>[4x]MNYGITESVKTTRSKIKIKDIVSDVVEKKANAIKYFLEGEEFKQAIVFGAYLSGSYIAYSLLKDCEEVIIVDIQPHLKDILFNDGIKFMDLNKLQLELRNGTSINPDLVIDLTGIGGVSPDLISKFNPKVLIVEDPKGNHDKGISKIDNTDKRLCVGAKKGV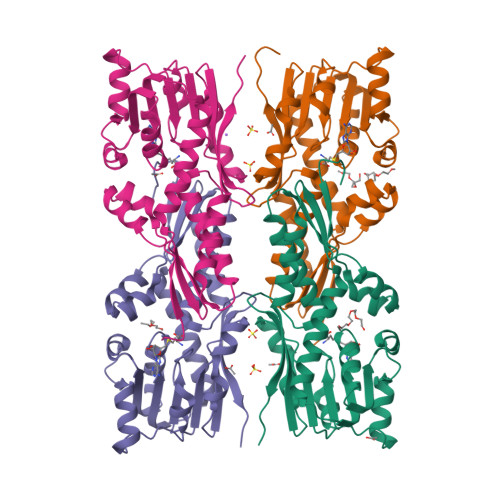LKTYRSSKFSKTSGTMTLVVDIIMDSCREINELDSVLYTIPNLKYFEGTVFHEKNVKKFLTELNMSAITVSSIDHVEYELEEILSKNISRVDSFVKEFDKLAAALEHHHHHH>TTTILGFKISMPIMIAPTAMQKMAHPEGEYATARAASAAGTIMTLSSWATSSVEEVASTGPGIRFFQLYVYKDRNVVAQLVRRAERAGFKAIALTVWKDVAWLQTITSLPILVKGVITAEDARLAVQHGAAGIIVSNHGARQLDYVPATIMALEEVVKAAQGRIPVFLDGGVRRGTDVFKALALGAAGVFIGRPVVFSLAAEGEAGVKKVLQMMRDEFELTMALSG[6x];>[12x]HMLVLVAPGQGAQTPGFLTDWLALPGAADRVAAWSDAIGLDLAHFGTKADADEIRDTSVAQPLLVAAGILSAAALGTGFTPGAVAGHSVGEITAAVFAGVLDDTAALSLVRRRGLAMAEAAAVTETGMSALLGGDPEVSV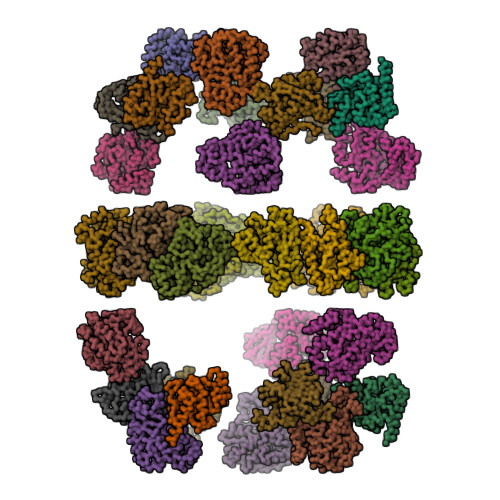AHLERLGLTPANVNGAGQIVAAGTMEQLAALNEDKPEGVRKVVPLKVAGAFHTRHMAPAVDKLAEAAKALTPADPKVTYVSNKDGRAVASGTEVLDRLVGQVANPVRWDLCMETFKELGVTAIIEVCPGGTLTGLAKRALPGVKTLALKTPDDLDAARELVAEHT;>MKRVVITGLGIVSSIGNNQQEVLASLREGRSGITFSQELKDSGMRSHVWGNVKLDTTGLIDRKVVRFMSDASIYAFLSMEQAIADAGLSPEAYQNNPRVGLIAGSGGGSPRFQVFGADAMRGPRGLKAVGPYVVTKAMASGVSACLATPFKIHGVNYSISSACATSAHCIGNAVEQIQLGKQDIVFAGGGEELCWEMACEFDAMGALSTKYNDTPEKASRTYDAHRDGFVIAGGGGMVVVEELEHALARGAHIYAEIVGYGATSDGADMVAPSGEGAVRCMKMAMHGVDTPIDYLNSHGTSTPVGDVKELAAIREVFGDKSPAISATKAMTGHSLGAAGVQEAIYSLLMLEHGFIAPSINIEELDEQAAGLNIVTETTDRELTTVMSNSFGFGGTNATLVMRKLKD[6x];>SPVVVVTGASRGIGKAIALSLGKAGCKVLVNYARSAKAAEEVSKQIEAYGGQAITFGGDVSKEADVEAMMKTAIDAWGTIDVVVNNAGITRDTLLIRMKKSQWDEVIDLNLTGVFLCTQAATKIMMKKRKGRIINIASVVGLIGNIGQANYAAAKAGVIGFSKTAAREGASRNINVNVVCPGFIASDMTAKLGEDMEKKILGTIPLGRTGQPENVAGLVEFLALSPAASYITGQAFTIDGGIAI[6x];>[6x]AIGQKLPPFSYAYTELEAIMYALGVGASIKDPKDLKFIYEGSSDFSCLPTFGVIIGQKSMMVLHGEQYLELYKPLPRAGKLKCEAVVADVLVVIIMDVYSYSEKELICHNQFSLFLSDKVKVAVAIPNRPPDAVLTDTTSLNQAALYRLSGDWNPLHIDPNFASLAGFDKPILHGLCTFGFSARRVLQQFADNDVSRFKAVKARFAKPVYPGQTLQTEMWKEGNRIHFQTKVQETGDIVISNAYVDLA Viruses from the family Picornaviridae form non-enveloped icosahedral virions that are about 30 nm in diameter. The capsid proteins VP1, VP2, VP3, and VP4 originating from a single polyprotein form a protomer, the basic building block of the icosahedral capsid. The entire capsid consists of 60 such protomers, arranged in 12 pentamer units. Here we show that the exit of the RNA from the particles of echoviruses 18 and 30 requires capsid opening and results in a loss of up to three adjacent capsid protein pentamers.

Specifically, we performed cryo-EM of echovirus 18 virions exposed to pH 6.0 for 10 min, mimicking the acidic environment that the virus encounters in endosomes. Asymmetric reconstruction combined with 3D classification identified subpopulations of echovirus 18 particles that lacked up to three pentamers of capsid protein protomers. We call the particles lacking one or several pentamers open particles. The missing pentamers always formed a single compact opening through the capsid. Reconstructions of the open particles missing one, two, or three pentamers with imposed five-fold, two-fold, and three-fold symmetries, respectively, were determined to resolutions of 3.8, 4.1, and 3.7 Å, which allowed their molecular structures to be built. Except for the missing pentamers, the open particles are similar in structure to that of the activated echovirus 18 particle: increased diameter relative to the native virus, reduced inter-pentamer contacts, absence of VP4 subunits, and holes along icosahedral two-fold symmetry axes. The capsid proteins next to the missing pentamers are more mobile than the rest of the capsid, as indicated by the three times higher temperature factors than the remainder of the capsid. Residues 1–42 from the N termini of VP1 subunits, which were previously shown to interact with membranes and facilitate enterovirus genome delivery into the cytoplasm, are not resolved in the electron density map, indicating that their structures differ among particles. The N-termini of some of the VP1 subunits could reach out of the capsid through the openings formed by the missing pentamers. The openings formed by the removal of one or more pentamers are sufficiently large to allow release of the viral RNA, even if the genome contains double-stranded RNA segments.

>[15x]GDNQDRTVANTQPSGPSNSTEIPALTAVETGHTSQVDPSDTIQTRHVVNFHSRSESTIENFMGRAACVFMDQYKINGEETSTDRFAVWTINIREMAQLRRKCEMFTYMRFDIEMTMVITSCQDQGTILDQDMPVLTHQIMYVPPGGPIPAKVDGYEWQTSTNPSVFWTEGNAPPRISIPFISVGNAYSSFYDGWSHFTQDGTYGYTTLNAMGKLYIRHVNRSSPHQITSTIRVYFKPKHIKAWVPRPPRLCPYINKRDVNFVVTEITDSRTSITDTPHPEHSVLATH;>[15x]SPSAEECGYSDRVRSMTLGNSTITTQESANVVVGYGEWPSYLSDREATAEDQPTQPDVATCRFYTLESVQWEKTSPGWWWKFPEALKNMGLFGQNMHYHYLGRAGYTIHVQCNASKFHQGCLLVVCVPEAEMGCADTDTTFPATELTTEDTPHVFTSDSITGKKVQAAVCNAGMGVGVGNLTIFPHQWINLRTNNSATIVIPYINSVPMDNMFRHYNFTLMIIPFAPLNFTDGATAYVPITVTIAPMYAEYNGLRLASTQ;>[15x]GVPVLNTPGSNQFLTSDDYQSPSAMPQFDETPEMHIPGEVRNLMEIAEVDSVVPVNNVTGKTKSMDAYQIPVGTGNTDKTKPIFSFQMDPGYSSVLKRTLLGEMLNYYAHWSGSVKLTFLFCGSAMATGKLLISYSPPGASVPTSRKDAMLGTHIVWDIGLQSSCVLCVPWISQSHYRMVQQDPYTSAGYITCWYQTNIVVPPGAPTSCDVLCFASACNDFSVRLLRDTPFMAQPGKLQ>SPRPFNEIPSPGDNGWLNLYHFWRETGTHKVHLHHVQNFQKYGPIYREKLGNVESVYVIDPEDVALLFKSEGPNPERFLIPPWVAYHQYYQRPIGVLLKKSAAWKKDRVALNQEVMAPEATKNFLPLLDAVSRDFVSVLHRRIKKAGSGNYSGDISDDLFRFAFESITNVIFGERQGMLEEVVNPEAQRFIDAIYQMFHTSV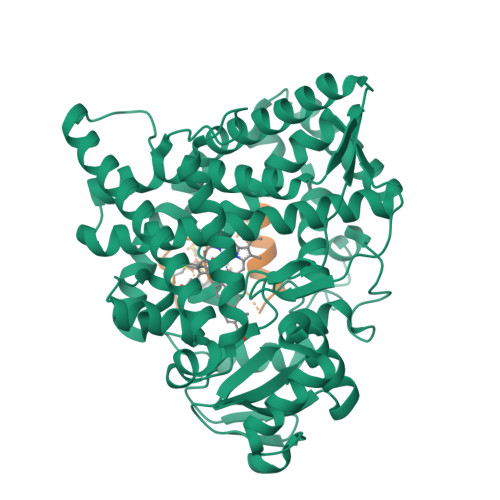PMLNLPPDLFRLFRTKTWKDHVAAWDVIFSKADIYTQNFYWELRQKGSVHHDYRGILYRLLGDSKMSFEDIKANVTEMLAGGVDTTSMTLQWHLYEMARNLKVQDMLRAEVLAARHQAQGDMATMLQLVPLLKASIKETLRLHPISVTLQRYLVNDLVLRDYMIPAKTLVQVAIYALGREPTFFFDPENFDPTRWLSKDKNITYFRNLGFGWGVRQCLGRRIAELEMTIFLINMLENFRVEIQHLSDVGTTFNLILMPEKPISFTFWPF[2x];>[2x]SLLDVVVENNLDIDGFGACEGTLACSTCHLIFEDHIYEKLDAITDEENDMLDLAYGLTDRSRLGCQIC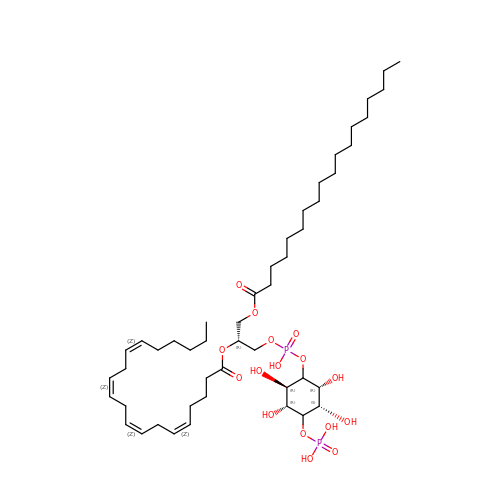(2R)-1-{[(R)-hydroxy{[(1R,2R,3R,4R,5S,6R)-2,3,5,6-tetrahydroxy-4-(phosphonooxy)cyclohexyl]oxy}phosphoryl]oxy}-3-(octadecanoyloxy)propan-2-yl (5Z,8Z,11Z,14Z)-icosa-5,8,11,14-tetraenoate | C47 H84 O16 P2 | ROKMWIUSHIHOGI-BWTMTLBLSA-N>SIHTKLRKSSRGFGFTVVGGDEPDEFLQIKSLVLDGPAALDGKMETGDVIVSVNDTCVLGHTHAQVVKIFQSIPIGASVDLELCR[2x];>RRRETQ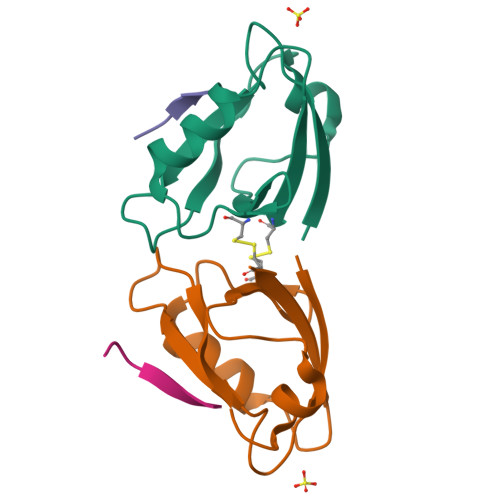V[2x]>[2x]LKCYSSRTETMTCPEGEDKCEKYAVG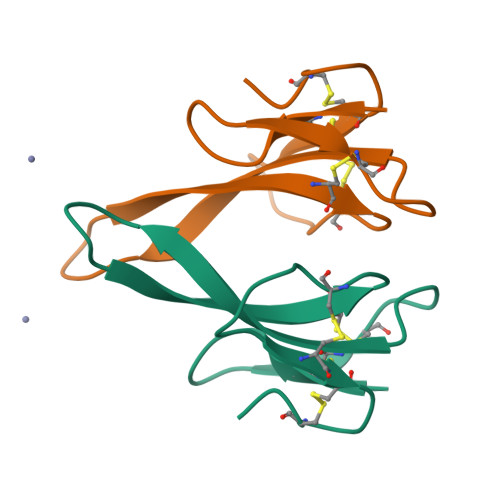LMHGSFFFIYTCTSKCHEGAYNVCCSTDLCNK>[2x]TFDERVAEVFPDMIQRSVPGYSNIISMIGMLAERFVQPGTQVYDLGCSLGAATLSVRRNIHHDNCKIIAIDNSPAMIERCRHHIDAYKAPTPVDVIEGDIRDIAIENA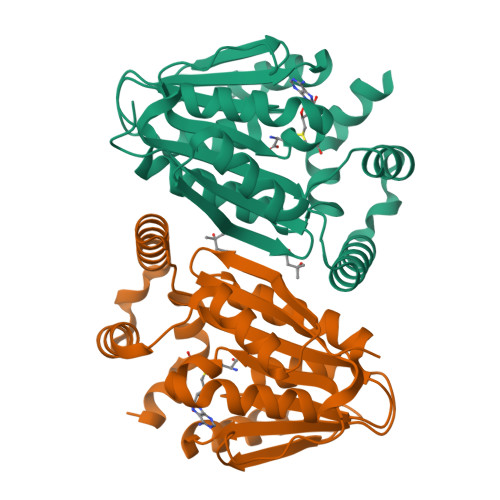SMVVLNFTLQFLEPSERQALLDKIYQGLNPGGALVLSEKFSFEDAKVGELLFNMHHDFKRANGYSELEISQKRSMLENVMLTDSVETHKARLHNAGFEHSELWFQCFNFGSLVALKAEDAA> METPLDLLKLNLDERVYIKLRGARTLVGTLQAFDSHCNIVLSDAVETIYQLNNEELSESERRCEMVFIRGDTVTLISTPSEDDDGAVEIWSHPQFE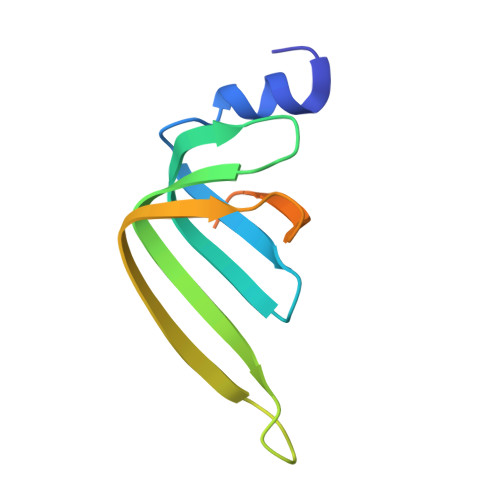K> GTAGLPRRIIKETQRLLAEPVPGIKAEPDESNARYFHVVIAGPQDSPFEGGTFKLELFLPEEYPMAAPKVRFMTKIYHPNVDKLGRICLDILKDKWSPALQIRTVLLSIQALLSAPNPDDPLANDVAEQ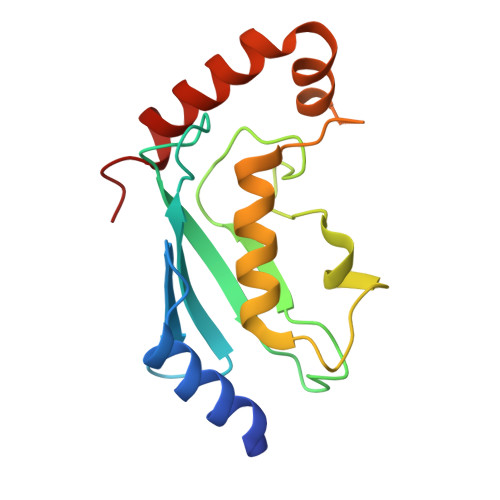WKTNEAQAIETARAWTRLYAMNNI3,4-dimethoxybenzoic acid | C9 H10 O4 | 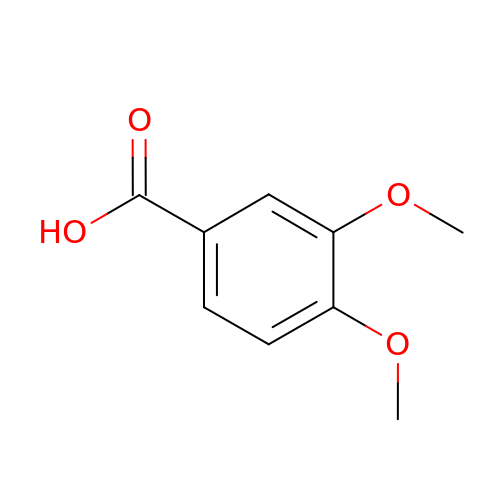DAUAQNGYDSHRET-UHFFFAOYSA-N>VLRKLKSGLERGLDTFDSTIEIIMQNLKTELESRCSDEVVEQQETENFLEQLISRIFQVVSRLTGVRIRNVQVPDITMEATSENSANVLIPITADVTVSLPFLGEIVDLDLNVDLQTTVSIETDTED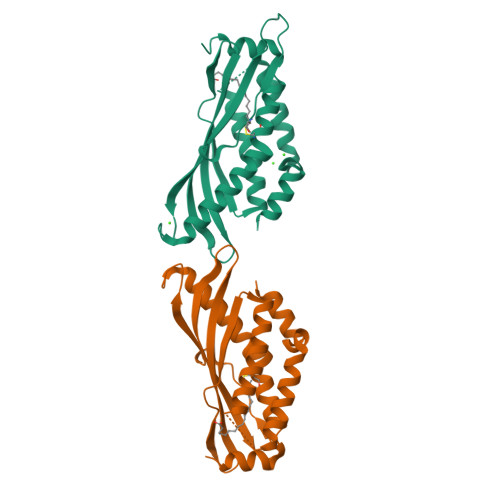PQVVVGECTNNPESISLTVLHSRFGLVNDVVDIGVNLARRVVSSVVEGELCPRFRELLESLDAECVEKLIGESQ[2x]>[18x]GFFSFIGEAFQGAGDMWRAYTDMKEAGW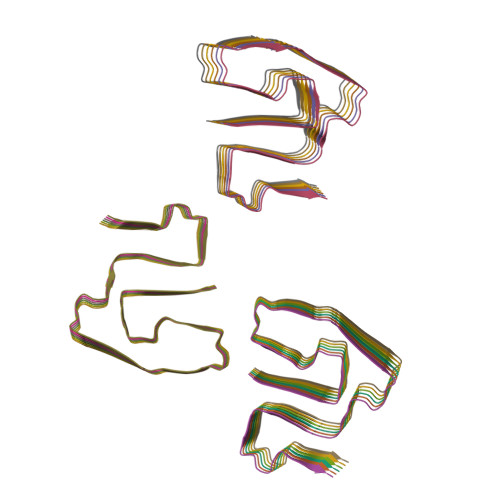KDGDKYFHARGNYDAAQRGPGGVWAAEKISDARESFQEFFGRGHEDTMADQEANR>MTEEHVVYIGKKPVMNYVLAVITQFHEGAKEVSIKARGRAISRAVDVAEIVRNRFLKDDVDVKEIKIGTEELPTADGRTTNTSTI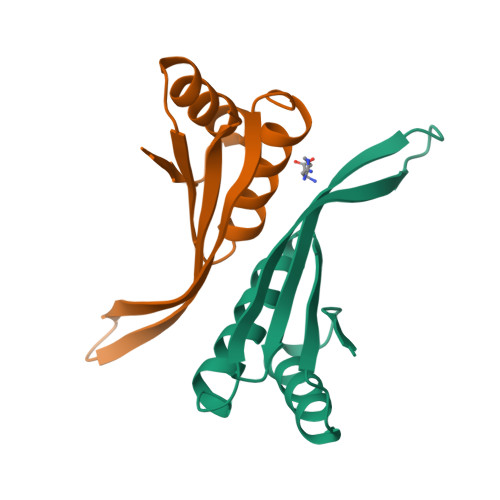EIVLARKT[4x]> AWATEQKTEEIPPPDLYKDTPAWYQAVYKDNVGLSEGSGPFTKYFKAQMLDMYWQPNRHYEPMENLDHSIFIEQERRDLCVICHEEATPGIVADWRSSGHKHPKSTPYLSSKTAQIEKNVGRVLDEVHCFDCHADTEKNQIRMPTGEVCGGCHRQQFDEFLREREVGRPNHLQSWEANTIVPWYAEAARRGYLYGQHGCDMCHSGAEKCDVCHTRHKFSAVEGRQPEACMTCHMGPDHPDAESYGESKHGKIYEKEEEHYDFTKPLVEVRPGEDYRTPTCQYCHMYEKHGRFIHNPVMKGIWRMGTVPPSNLEYTSSLKDYPYGIKIIADKIDIYSEENVAKRSYWLEVCAKCHSDRFADTYLKSLDQFMFQAHTLADQAQKIVEDLIADGLLYPDAAN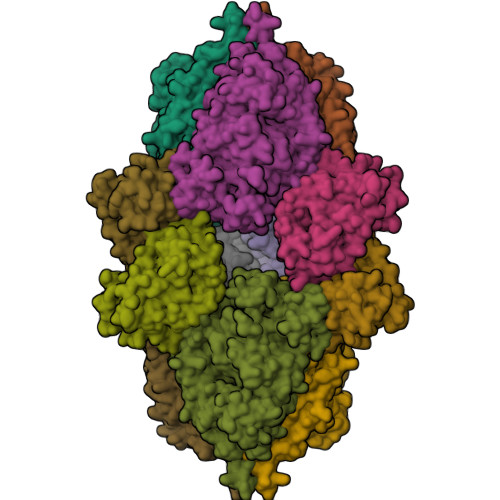RDPYPLSDGIVKELSADFLGEPVYNAFKTLQGKFPVVGPILGVYGMFLQMQDNPSDIENMYNRLWFWYKLQGYKGTAHAQQDVSWWWGQAPMMMEMTRIQAEAARLRRLAGIEKTISK;> IEIPKEVTEEGKNVYKKYCAPCHGEEGGGDGLLSRSMLPKPRNFTLGAYKFRTTPSGSLPTDEDIYRTISYGVPNSTMIPWDILTEEQRASVVPVLKSFSEAFEYREPEPSVDVGLPLRPTERTILAGKKIYEEKLECWKCHGVEGRGDGPSASEQEDDFGFPIKPFDFTTGKFKGGNSPTDVYLRFTTGLNGTPMPSFAKELSDDERWYLTHYVMSLVQPEKCRK>GAMGEQIFYWSPAKHWRMSDEGVVIGESTYTGMILEWFPEFYFFAQTGVTINRLLERFSSGSEKEANEILELLIQDRVLVEGILPPREVFSPQEGLFVNPYSEQIRYSKEALDYYVSEQLNRTHAACRSTKIQLETSGALPDIIQKRRSCRRFDMKTPVSFATFSNLLSSLKQRKEDKILYNYASAGGLYPIDVFVYVKPRRVEGVKAGFYYFNPADHSLVLVNNIDQVIKDDHELINQDIFAQSAFSVYLVYNARASMPKYGAAGYFYACIEAGIITATLNMVAEDLNVGLCSIGHMNFEEIQTFLKLEDHQVILHAIEGGLKIDGAAAENLYFQ[2x];> GAMEADLSEPFSLTEVQTAYMLGRNPQFELSGISPQTYFEYETELDIARLSRSFQKVIQRHPMLRAVILPEGKQQILRDVPEYEIEVESLVSMPPEKQAARLREERSRMIDHVFPLGQWPLFELKAFQLQEHTYLLCFRYDALLMDGASMNLVGQDLMHYYHQPDAQLPPLSFTFQDYMHIYDDMKRGTEYETAKAYWTNKLPDFPPAPSLLLAKDPAEIGTPNFQSLTTIITKDKWLKLRRLAQDKQVTPSALLCTVYGEVLAFWSNQRRLAINLTVFNRYPVHDEVEQIVGDFTSLILLDMDMDQKQPFFTKVEQTQSTLLDGLEHRHYDGVEFIRDYTRYHQMRPKAVMPIVFTSMLAGAGAFAWEEIGSLRHIHARTPQVYLDNVVIEKNGELLVSWNYVEELFDAEVMESMFTQFVELLDQLVEQGDINPLRISQKDYALIDQYNATAEPIPAATLHQLFIDQAQRTPDQVAVVFEQEWLTYSELDQRSNQVARFLQSRGIGRGDRVGVLAKRQVETIINLMAVLKAGAAYVPIDPDHPYERQTYILENSSCKILLDSDLYETMEISSYADGDLTPVAEPEDTAYVIYTSGSTGRPKGVIITHQAASNTIQDINRKFEVNEEDRIIGISSMCFDLSVYDIFGTLSAGATLVMIRDPRDMRELVRTVERRGITIWNTVPAIMDLALDHVGSHFENISLRLVLLSGDWIPLPLPAKINRHFPVADVISLGGATEASIWSIYWPIEQVEANWKSIPYGKPLANQTYYVLNYDQKMCPVGVIGDLYIGGAGLAQGYLNDDQKTKDAFIMHPEFGPIYKTGDCGRMRPEGYIEFLGRQDYQVKIQGYRVELEEISHCLLTYPDVDQAVVIDQTDERGMKFLVGYVVAQQEIDEKALRKHLMEHLPEYMIPAHLVHLEQLPLTPNGKLDRKALPVPKKQRNAEKFVAPQAGLEKILASVWQEVLNVEQI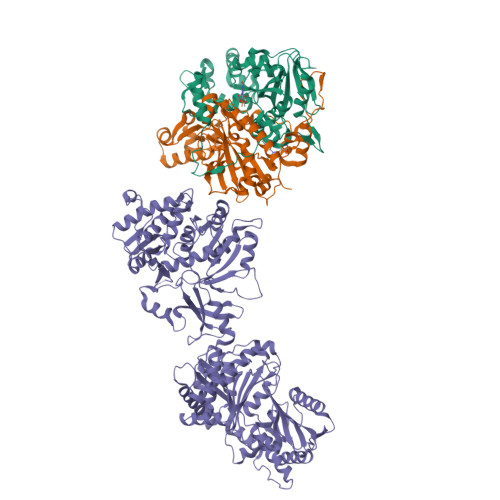GANDHFFALGGDSIKAIQVSARLFVQGYHLDTKSLFEFPVLRDVARTIKKLAAAENLYFQ>[3x]ATPHINAEMGDFADVVLMPGDPLRAKYIAETFLEDAREVNNVRGMLGFT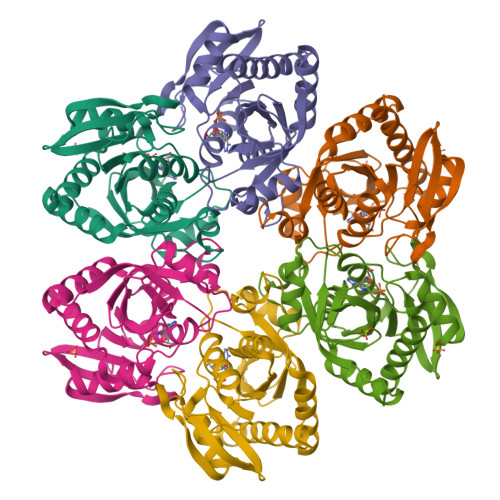GTYKGRKISVMGHGMGIPSCSIYTKELITDFGVKKIIRVGSCGAVLPHVKLRDVVIGMGACTDSKVNRIRFKDHDFAAIADFDMVRNAVDAAKALGIDARVGNLFSADLFYSPDGEMFDVMEKYGILGVEMEAAGIYGVAAEFGAKALTICTVSAHIRTHEQTTAAEAQTTFNDMIKIALESVLLGDK>[3x]GSRTDLLNVCMDAKHHKTKPGPEDKLHDQCSPWKKNACCTASTSQELHKDTSRLYNF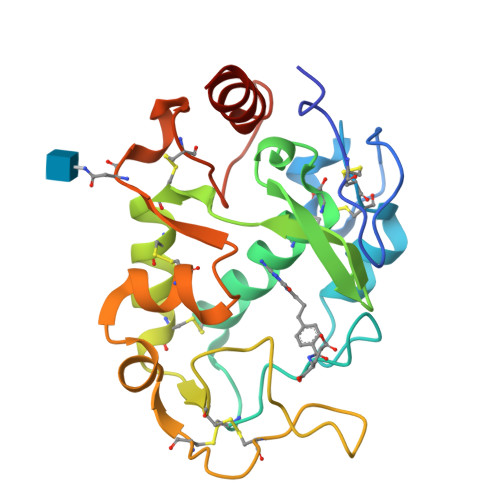NWDHCGKMEPACKRHFIQDTCLYECSPNLGPWIQQVNQSWRKERFLDVPLCKEDCQRWWEDCHTSHTCKSNWHRGWDWTSGVNKCPAGALCRTFESYFPTPAALCEGLWSHSYKVSNYSRGSGRCIQMWFDSAQGNPNEEVARFYAAAMH>AEAGITGTWYNQLGSTFIVTAGADGALTGTYESAVGNAESRYVLTGRYDSAPATDGSGTA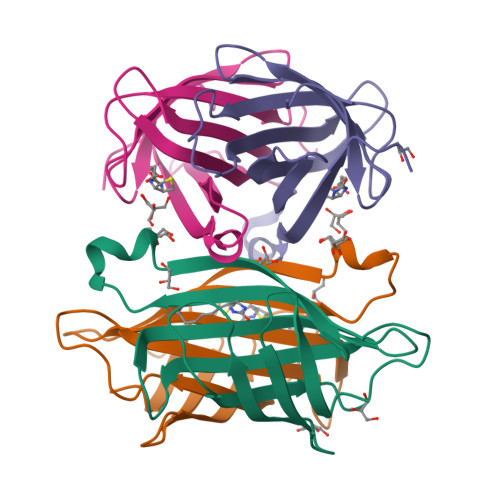LGWTVAWKNNYRNAHSATTWSGQYVGGAEARINTQWLLTSGTTEANAWKSTLVGHDTLTKVKPSAAS[4x]>MASMKKSTENESTNYQYKIQELR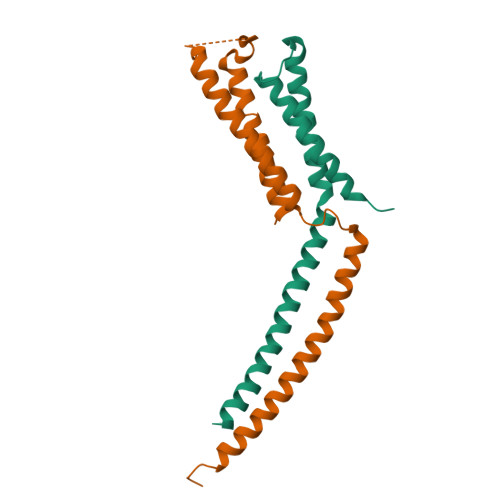KLLKSLLLNYLELIGVLSINPDMYERKVENIRTILVNIHHLLNEYRPHQSRESLIMLLEEQLEYKRGEIREIEQVCKQVHDKLTS[2x];>[2x]MTDRLTQLQICLDQMTEQFCATLNYIDKNHGFERLTVNEPQMSDKHATVVPPEEFSNTIDELSTDIILKTRQINKLIDSLPGVDVSAEEQLRKIDMLQKKLVEVEDEKIEAIKKKEKLLRHVDSLIEDFVDGIANSKKSTAAALEHHHHHH>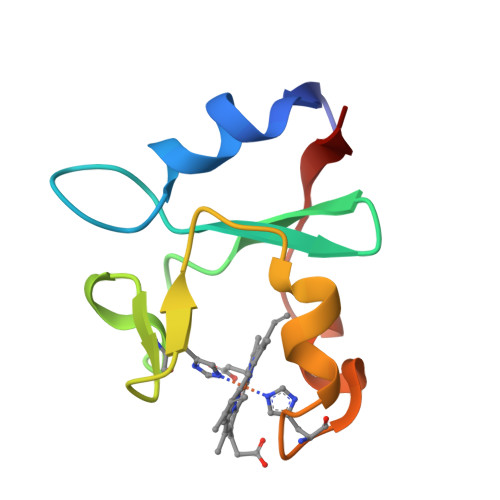 AMEEFTTEELAKYNGKDGEKCYFAYKGKVYDVTESMLWEDGDHQGMHEGGIDLTADHEDAPHDDDVLEDFPVVGTLKA> GPEKEWVEQDEP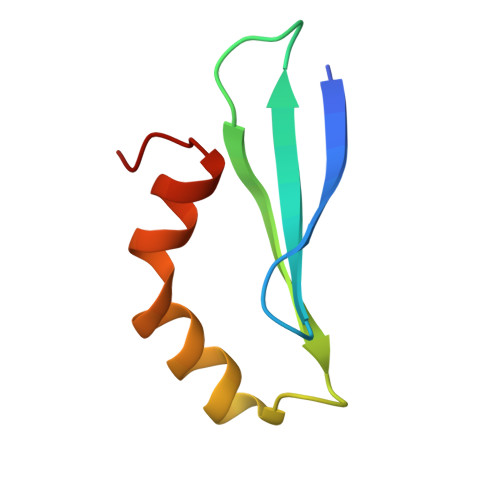GVYITLTALAGGARDLKRVRFSRKRFSEIQAEQWWADNRGRVYEQYNVRMV>[6x]MDALELLVNRRSASR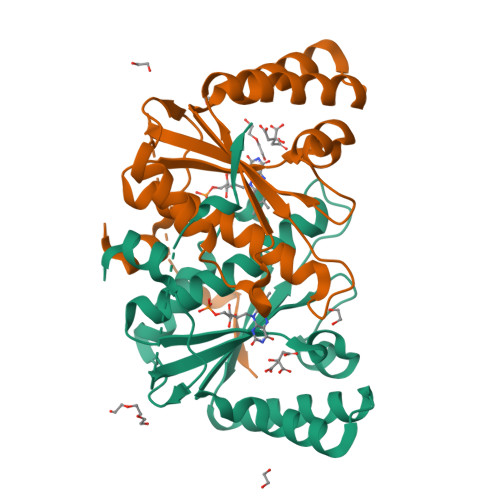LAEPAPVGEQLQNILRAGMRVPDHKSLQPWRFFVIEGEGRDRFSAVLEQGAVAAGGDEKAIEKARNAPFRAPLIITVVAKCEENHKVPVWEQEMSAGCAVMAMQMAAIAQGFNGIWRSGALTESAIVREAFECRPQDKIVGFLYLGTPQLKASTTISTPDPTPFVRYF> EAPHLVQVDA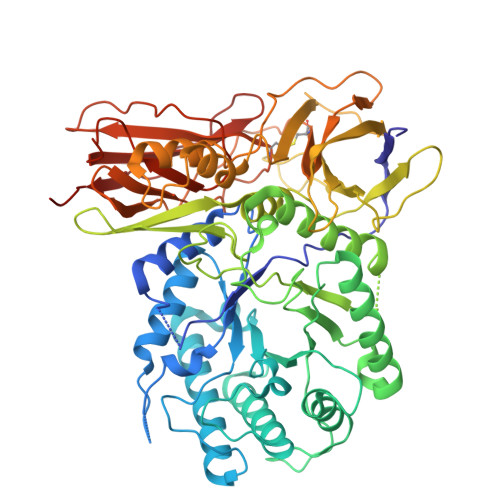ARALWPLRRFWRSTGFCPPLPHSQADPYVLSWDQQLNLAYVGAVPHRGIKQVRTHWLLELVTTRGSTGQGLSYNFTHLDGYLDLLRENQLLPGFELMGSASGHFTDFEDKQQVFEWKDLVSSLARRYIGRYGLAHVSKWNFETWNEPDHHDFDNVSMTMQGFLNYYDACSEGLRAASPALRLGGPGDSFHTPPRSPLSWGLLRHCHDGTNFFTGEAGVRLDYISLHRKGARSSISILEQEKVVAQQIRQLFPKFADTPIYNDEADPLVGWSLPQPWRADVTYAAMVVKVIAQHQNLLLANTTSAFPYALLSNDNAFLSYHPHPFAQRTLTARFQVNNTRPPHVQLLRKPVLTAMGLLALLDEEQLWAEVSQAGTVLDSNHTVGVLASAHRPQGPADAWRAAVLIYASDDTRAHPNRSVAVTLRLRGVPPGPGLVYVTRYLDNGLCSPDGEWRRLGRPVFPTAEQFRRMRAAEDPVAAAPRPLPAGGRLTLRPALRLPSLLLVHVCARPEKPPGQVTRLRALPLTQGQLVLVWSDEHVGSKCLWTYEIQFSQDGKAYTPVSRKPSTFNLFVFSPDTGAVSGSYRVRALDYWARPGPFSDPVPYLEVPVPRGPPSPGNP>MLALGIEGTAHTLGIGIVSEDKVLANVFDTLTTEKGGIHPKEAAEHHARLMKPLLRKALSEAGVSLDDIDVIAFSQGPGLGPALRVVATAARALAVKYRKPIVGVNHCIAHVEITKMFGVKDPVGLYVSGGNTQVLALEGGRYRVFGETLDIGIGNAIDVFARELGLGFPGGPKVEKLAEKGEKYIELPYAVKGMDLSFSGLLTEAIRKYRSGKYRVEDLAYSFQETAFAALVEVTERAVAHTEKDEVVLVGGVAANNRLREMLRIMTEDRGIKFFVPPYDLCRDNGAM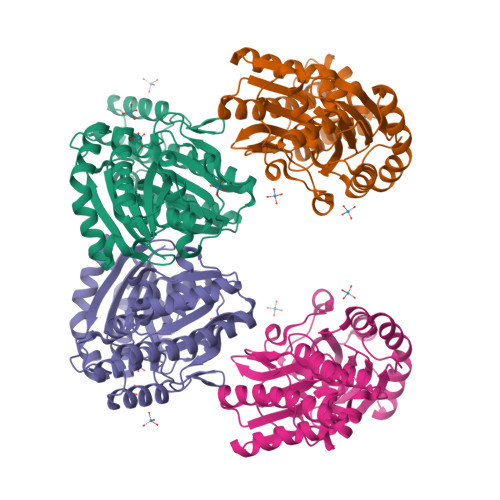IAYTGLRMYKAGISFRLEETIVKQKFRTDEVEIVWHHHHHH[4x]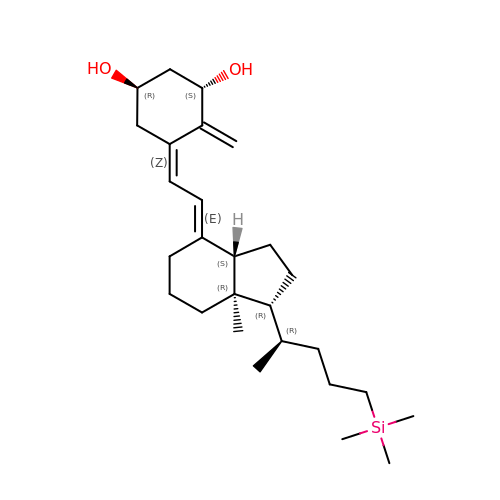(1~{R},3~{S},5~{Z})-5-[(2~{E})-2-[(1~{R},3~{a}~{S},7~{a}~{R})-7~{a}-methyl-1-[(2~{R})-5-trimethylsilylpentan-2-yl]-2,3,3~{a},5,6,7-hexahydro-1~{H}-inden-4-ylidene]ethylidene]-4-methylidene-cyclohexane-1,3-diol | C27 H46 O2 Si | OTBSZBXRIBUUEI-AVJTYSNKSA-N> VEIPSSFDSRKKWPRCKSIATIRDQSRCGSCWAFGAVEAMSDRSCIQSGGKQNVELSAVDLLSCCESCGLGCEGGILGPAWDYWVKEGIVTGSSKENHAGCEPYPFPKCEHHTKGKYPPCGSKIYKTPRCKQTCQKKYKTPYTQDKHRGKSSYNVKNDEKAIQKEIMKYGPVEAGFTVYEDFLNYKSGIYKHITGETLGGHAIRIIGWGVENKAPYWLIANSWNEDWGENGYFRIVRGRDECSIESEVTAGRIN

The component digestive proteases in Schistosoma mansoni (S. mansoni) include the CA clan cysteine proteases, cathepsin B1, cathepsin C (dipeptidyl aminopeptidase I), and cathepsins L1–L3, the CD clan protease known as legumain (asparaginyl endopeptidase), and the clan AA aspartic protease, cathepsin D.11,13,14S. mansoni cathepsin B1 (SmCB1) is a central digestive protease due to its high abundance and dual mode of action as both an endo- and an exopeptidase (specifically, a carboxydipeptidase). This dual activity is enabled by the flexible occluding loop that restricts access to the active site. The occluding loop is characteristic of cathepsin B-type proteases and distinguishes them from cathepsin L-type proteases, which are strict endopeptidases. The inhibitors are located in the active site cleft of SmCB1, which contains the catalytic residues Cys100 and His270 (supported by Asn290 and Gln94) and has restricted access to the primed region (beyond S1′ and S2′ subsites) by the occluding loop (Phe175 to Pro197), a hallmark of cathepsins B.15,17 Gallinamides form an irreversible covalent bond to the thiol group of Cys100 through the Cß atom of the vinyl group of the acrylamide warhead.

The structures were determined by molecular replacement and refined using data to resolutions of 1.20 1.60, and 1.55 Å for the complexes of gallinamide A, 1, and 6, respectively. The P1′ position contains the C-terminal MMP group with various R1′ substituents, including side chains of alanine, leucine, and phenylalanine in gallinamide A, 1, and 6, respectively. Two different conformations were modeled for the phenylalanine side chain in the MMP group of compound 6. In one conformation (labeled A in Figure 4), it is flipped out from the S1′ subsite to S1, while in the other (B), it is directed toward the S2′ subsite. The conformation A appears to be intramolecularly stabilized by a CH-π interaction of the P1′-phenylalanine and P1 alanine side chains. Each conformation is associated with a different orientation of the methoxy group on the MMP ring and a different conformation of His181 on the occluding loop in S2′. A double conformation of Ile193 was observed in the complexes of 1 and gallinamide A, but not in the complex of 6 due to steric hindrance by R1′. However, for 6, we observed a T-shape π–π interaction of the MMP ring in conformation A with Trp292. Not surprisingly, P4 is not involved in significant interactions with SmCB1, except for a hydrophobic interaction of the P4 phenylalanine of 6, which is rotated to approach Leu139 in the S3 subsite.> MGIPTEVTLPVEVHDAQFVDFRANSGTSDVWVQHEGSSAGFGDVGSSGDNAFGDGGSARVRFKKDVFNHDFSALPGVSQVVEGLPFNTDVTYSLYYCD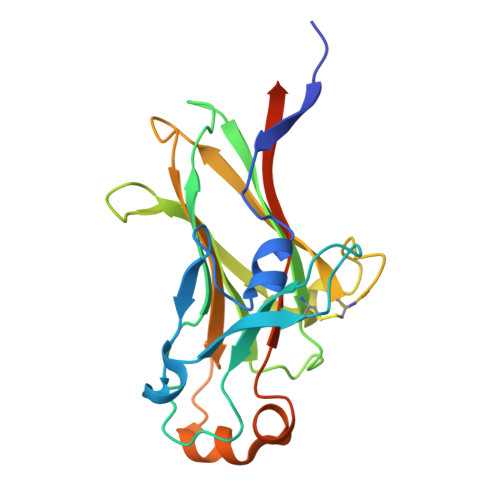NKKDDSLSTLYFGARDINGNAITEEYAHVKDLSNAPQGTNKTCFKKVSTTFNTGNNGSVELFALMAIDVNGTMTEEEIYASSQFTSNELEVRLDEFSLTYKGEASDELLEHHHHHH>[4x]MKKLIVDLDGTLTQANTSDYRNVLPRLDVIEQLREYHQLGFEIVISTARNMRTYEGNVGKINIHTLPIITEWLDKHQVPYDEILVGKPWCGHDGFYIDDRAVRPSEFASMNLEEIHQLFEKE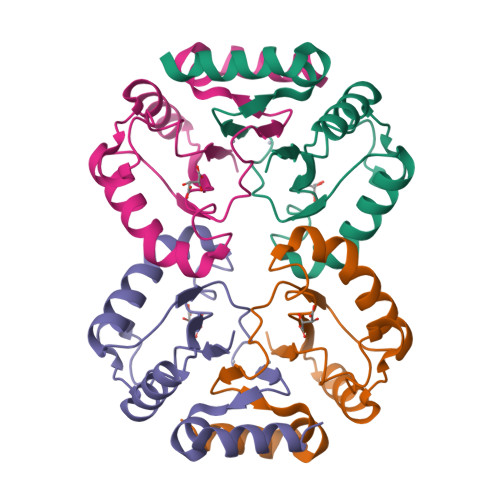KSCS>[2x]GPGSMNATLIDCCDPQKPSRVLFHFLILDAPSPSNLPTYIKELQHRGVRHLVRVCGPTY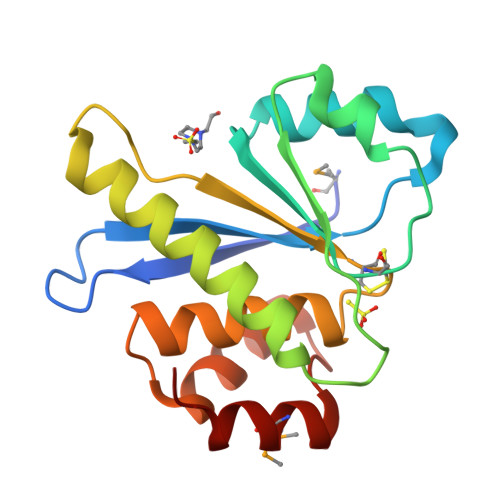DATLVKSRGIDVHSWPFDDGAPPTRAVLDSWLKLLDTELARQQEDPSVPPPTIGVHCVAGLGRAPILVALALVEYGNVSALDAIALIREKRKGAINQTQMHWITKYKR> TVGAVALDLDGNLAAATSTGGMTNKLPHTVGPQPLVGAGCYANNASVAVSCTGTGEVFIRALAAYDIAALMDYGGLSLAEACERVVMEKLPALGGSGG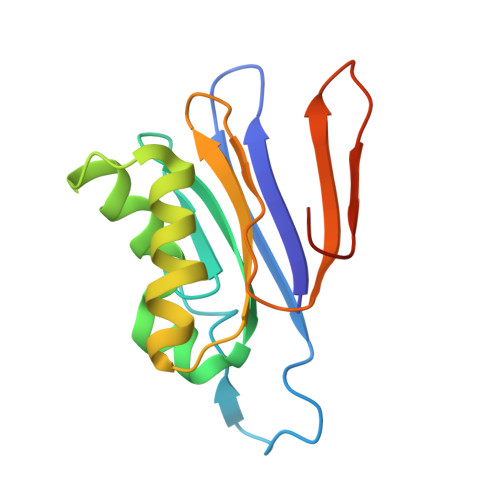LIAIDHEGNVALPFNTEGMYRAWGYAGDTPTTGIYREKGDTVATQ N-HYDROXY-2-[2-(TRIFLUOROMETHYL)PHENYL]-1,3-OXAZOLE-4-CARBOXAMIDE 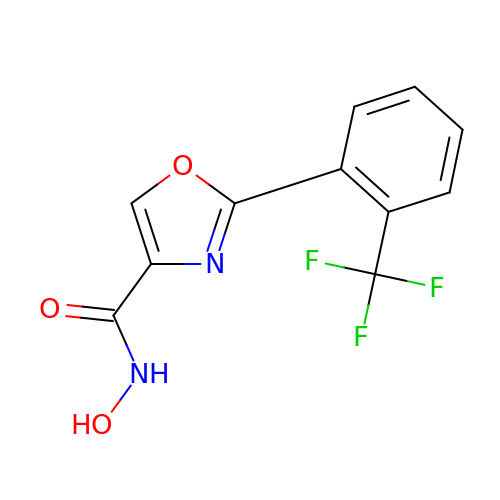| C11 H7 F3 N2 O3 | CRHXDKPGVAVHNT-UHFFFAOYSA-N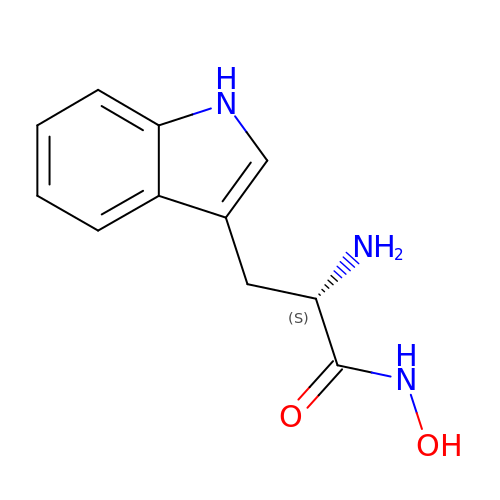N-hydroxy-L-tryptophanamide | C11 H13 N3 O2 | LBMAEBPZXXNKMZ-VIFPVBQESA-N>[2x]MNIVVLISGNGSNLQAIIDACKTNKIKGTVRAVFSNKADAFGLERARQAGIATHTLIASAFDSREA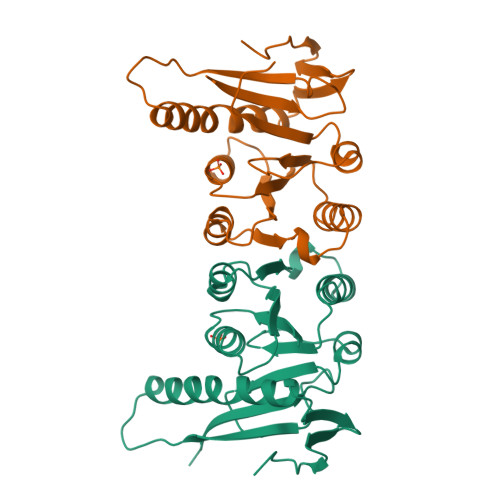YDRELIHEIDMYAPDVVVLAGFMRILSPAFVSHYAGRLLNIHPSLLPKYPGLHTHRQALENGDEEHGTSVHFVTDELDGGPVILQAKVPVFAGDSEDDITARVQTQEHAIYPLVISWFADGRLKMHENAAWLDGQRLPPQGYAADE KtrAB is a cation channel with a nucleotide-dependent RCK domain. The structure of the KtrAB complex revealed a homodimeric membrane protein (KtrB) assembled with a cytosolic RCK octameric ring, formed by the KtrA protein. KtrA binds nucleotides, ATP or ADP. ATP binding induces the adoption of a square-conformation by the octameric ring and increased K+ flux activity through KtrAB; ADP binding results in a non-square conformation and decreased flux.

We introduced the single-point mutations R16A, R16K, A80P and E125Q in KtrA and tested their impact in the complementation assay. However, and contrary to our predictions, none of the R16 mutations had an impact on the growth phenotype, while E125Q resulted in an apparently inactive KtrAB. The structures of R16K (at 2.7 Å resolution) and R16A (at 3.4 Å resolution) with ATP are very similar to that of the previously determined wild-type KtrA-ATP (WT-ATP), adopting the square conformation. A simple indicator of ring conformation is the pair of distances (L1 and L2) separating the Cα of N38 residues located in opposite subunits across a ring face. In the ATP-bound rings, these distances are similar in the R16K (30.8/30.8 Å), R16A (29.9/29.9 Å) mutants and wild-type (30.0/30.0 Å) structures. KtrA mutants that show a wild-type protein function (R16K and R16A) are able to adopt a square conformation with ATP. Importantly, they also reveal that, while R16 does not play a major role in the mechanism, A80 and E125 are crucial residues in the adoption of this conformation. In contrast, KtrAR16AB-ATP is also active in the choline condition without added Mg2+.

>MGRIKNKQFAVIGLGAFGGSICKELHRMGHEVLAVDINEEKVNAYASYATHAVIANATEENELLSLGIRNFEYVIVAIGANIQASTLTTLLLKELDIPNIWVKAQNYYHHKVLEKIGADRIIHPEKDMGVKIAQSLSDENVLNYIDLSDEYSIVELLATRKLDSKSIIDLNVRAKYGCTILAIKHHGDICLSPAPEDIIREQDCLVIMGHKKDIKRFENEGM[2x]> LPDAPEFEKDLLIQRLNWMLWVIDECFRDLCYRTGICKGILEPAAIFHLKLPAINDTDHCGLIGFNETSCLKKLADGFFEFEVLFKFLTTEFGKSVINVDVM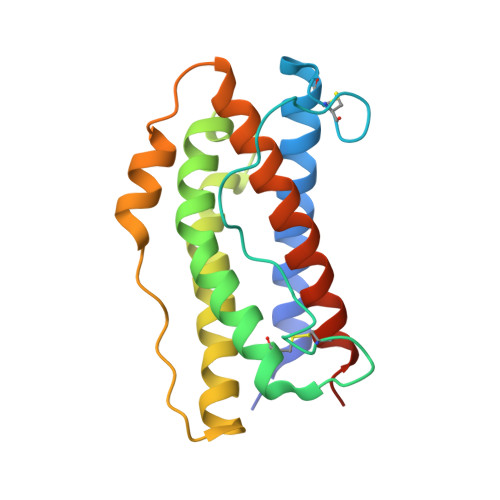ELLTKTLGWDIQEELNKLTKTHYSPPKFDRGLLGRLQGLKYWVRHFASFYVLSAMEKFAGQAVRVLDSIPDVTPDVHDK>[4x]MNLKDKILGVAKELFIKNGYNATTTGEIVKLSESSKGNLYYHFKTKENLFLEILNIEESKWQEQWKSEQIKCKTNREKFYLYNELSLTTQYYY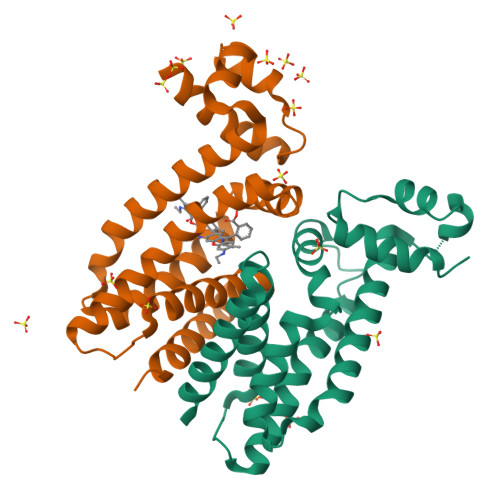PLQNAIIEFYTEYYKTNSINEKMNKLENKYIDAYHVIFKEGNLNGEWSINDVNAVSKIAANAVNGIVTFTHEQNINERIKLMNKFSQIFLNGLSKHHHHHH> MSILTRWLLIPPVNARLIGRYRDYRRHGASAFSATLGCFWMILAWIFIPLEHPRWQRIRAEHKNLYPHINASRPRPLDPVRYLIQTCWLLIGASRKETPKPRRRAFSGLQNIRGRYHQWMNELPERVSHKTQHLDEKKELGHLSAGARRLILGIIVTFSLILALICVTQPFNPLAQFIFLMLLWGVALIVRRMPGRFSALMLIVLSLTVSCRYIWWRYTSTLNWDDPVSLVCGLILLFAETYAWIVLVLGYFQVVWPLNRQPVPLPKDMSLWPSVDIFVPTYNEDLNVVKNTIYASLGIDWPKDKLNIWILDDGGREEFRQFAQNVGVKYIARTTHEHAKAGNINNALKYAKGEFVSIFDCDHVPTRSFLQMTMGWFLKEKQLAMMQTPHHFFSPDPFERNLGRFRKTPNEGTLFYGLVQDGNDMWDATFFCGSCAVIRRKPLDEIGGIAVETVTEDAHTSLRLHRRGYTSAYMRIPQAAGLATESLSAHIGQRIRWARGMVQIFRLDNPLTGKGLKFAQRLCYVNAMFHFLSGIPRLIFLTAPLAFLLLHAYIIYAPALMIALFVLPHMIHASLTNSKIQGKYRHSFWSEIYETVLAWYIAPPTLVALINPHKGKFNVTAKGGLVEEEYVDWVISRPYIFLVLLNLVGVAVGIWRYFYGPPTEMLTVVVSMVWVFYNLIVLGGAVAVSVESKQVRRSHRVEMTMPAAIAREDGHLFSCTVQDFSDGGLGIKINGQAQILEGQKVNLLLKRGQQEYVFPTQVARVMGNEVGLKLMPLTTQQHIDFVQCTFARADTWALWQDSYPEDKPLESLLDILKLGFRGYRHLAEFAPSSVKGIFRVLTSLVSWVVSFIPRRPERSETAQPSDQALAQQGSARSSGRTGLEFEEFYPYDVPDYAADYKDDDDKRS;>MKRKLFWICAVAMGMSAFPSFMTQATPATQPLINAEPAVAAQTEQNPQVGQVMPGVQGADAPVVAQNGPSRDVKLTFAQIAPPPGSMVLRGINPNGSIEFGMRSDEVVTKAMLNLEYTPSPSLLPVQSQLKVYLNDELMGVLPVTKEQLGKKTLAQMPINPLFITDFNRVRLEFVGHYQDVCENPASTTLWLDVGRSSGLDLTYQTLNVKNDLSHFPVPFFDPRDNRTNTLPMVFAGAPDVGLQQASAIVASWFGSRSGWRGQNFPVLYNQLPDRNAIVFATNDKRPDFLRDHPAVKAPVIEMINHPQNPYVKLLVVFGRDDKDLLQAAKGIAQGNILFRGESVVVNEVKPLLPRKPYDAPNWVRTDRPVTFGELKTYEEQLQSSGLEPAAINVSLNLPPDLYLMRSTGIDMDINYRYTMPPVKDSSRMDISLNNQFLQSFNLSSKQEANRLLLRIPVLQGLLDGKTDVSIPALKLGATNQLRFDFEYMNPMPGGSVDNCITFQPVQNHVVIGDDSTIDFSKYYHFIPMPDLRAFANAGFPFSRMADLSQTITVMPKAPNEAQMETLLNTVGFIGAQTGFPAINLTVTDDGSTIQGKDADIMIIGGIPDKLKDDKQIDLLVQATESWVKTPMRQTPFPGIVPDESDRAAETRSTLTSSGAMAAVIGFQSPYNDQRSVIALLADSPRGYEMLNDAVNDSGKRATMFGSVAVIRESGINSLRVGDVYYVGHLPWFERLWYALANHPILLAVLAAISVILLAWVLWRLLRIISRRRLNPDNE[4x];>[2x]MTQFTQNTAMPSSLWQYWRGLSGWNFYFLVKFGLLWAGYLNFHPLLNLVFAAFLLMPLPRYSLHRLRHWIALPIGFALFWHDTWLPGPESIMSQGSQVAGFSTDYLIDLVTRFINWQMIGAIFVLLVAWLFLSQWIRITVFVVAILLWLNVLTLAGPSFSLWPAGQPTTTVTTTGGNAAATVAATGGAPVVGDMPAQTAPPTTANLNAWLNNFYNAEAKRKSTFPSSLPADAQPFELLVINICSLSWSDIEAAGLMSHPLWSHFDIEFKNFNSATSYSGPAAIRLLRASCGQTSHTNLYQPANNDCYLFDNLSKLGFTQHLMMGHNGQFGGFLKEVRENGGMQSELMDQTNLPVILLGFDGSPVYDDTAVLNRWLDVTEKDKNSRSATFYNTLPLHDGNHYPGVSKTADYKARAQKFFDELDAFFTELEKSGRKVMVVVVPEHGGALKGDRMQVSGLRDIPSPSITDVPVGVKFFGMKAPHQGAPIVIEQPSSFLAISDLVVRVLDGKIFTEDNVDWKKLTSGLHKQHRSPRTQMQ;>MASWSHPQFEKGSMRDIVDPVFSIGISSLWDELRHMPAGGVWWFNVDRHEDAISLANQTIASQAETAHVAVISMDSDPAKIFQLDDSQGPEKIKLFSMLNHEKGLYYLTRDLQCSIDPHNYLFILVCANNAWQNIPAERLRSWLDKMNKWSRLNHCSLLVINPGNNNDKQFSLLLEEYRSLFGLASLRFQGDQHLLDIAFWCNEKGVSARQQLSVQQQNGIWTLVQSEEAEIQPRSDEKRILSNVAVLEGAPPLSEHWQLFNNNEVLFNEARTAQAATVVFSLQQNAQIEPLARSIHTLRRQRGSAMKILVRENTASLRATDERLLLACGANMVIPWNAPLSRCLTMIESVQGQKFSRYVPEDITTLLSMTQPLKLRGFQKWDVFCNAVNNMMNNPLLPAHGKGVLVALRPVPGIRVEQALTLCRPNRTGDIMTIGGNRLVLFLSFCRINDLDTALNHIFPLPTGDIFSNRMVWFEDDQISAELVQMRLLAPEQWGMPLPLTQSSKPVINAEHDGRHWRRIPEPMRLLDDAVERSS[2x];>[2x]MMTISDIIEIIVVCALIFFPLGYLARHSLRRIRDTLRLFFAKPRYVKPAGTLRRTEKARATKK;>[2x]MAVLGLQGVRGGVGTTTITAALAWSLQMLGENVLVVDACPDNLLRLSFNVDFTHRQGWARAMLDGQDWRDAGLRYTSQLDLLPFGQLSIEEQENPQHWQTRLSDICSGLQQLKASGRYQWILIDLPRDASQITHQLLSLCDHSLAIVNVDANCHIRLHQQALPDGAHILINNFRIGSQVQDDIYQLWLQSQRRLLPMLIHRDEAMAECLAAKQPVGEYRSDALAAEEILTLANWCLLNYSGLKTPVGSKS;>MGSSHHHHHHHHAAGSNNNEPDTLPDPAIGYIFQNDIVALKQAFSLPDIDYADISQREQLAAALKRWPLLAEFAQQK[2x]

Bacterial cellulosic polymers constitute a prevalent class of biofilm matrix exopolysaccharides that are synthesized by several types of bacterial cellulose secretion (Bcs) systems, which include conserved cyclic diguanylate (c-di-GMP)-dependent cellulose synthase modules together with diverse accessory subunits. In E. coli, the biogenesis of phosphoethanolamine (pEtN)-modified cellulose relies on the BcsRQABEFG macrocomplex, encompassing inner-membrane and cytosolic subunits, and an outer membrane porin, BcsC. Here we present cryo-EM structures of the E. coli Bcs macrocomplex positioning all seven BcsRQABEFG partners and multiple c-di-GMP-binding sites.

Here we locally refined the structure of the crownless Bcs macrocomplex complex to an average resolution of 2.85 Å, visualizing all interaction interfaces and coordinated nucleotide co-factors. An assymetric BcsR2Q2 complex is recruited to the membrane complex via BcsE’s C-terminal elongated tails, where both BcsQ copies interact with the synthase’s PilZ module and adopt the nucleotide-driven sandwich dimer conformation characteristic for the SIMIBI (SIgnal recognition particle, MinD, and BioD) family of protein-sorting NTPases to which BcsQ belongs. Importantly, whereas one of the BcsR protomers is solvent-exposed and features an unresolved N-terminal domain, the other BcsR copy also interacts with the back of the BcsA catalytic module. Contrary to the crystallized states where BcsRNTD can adopt a β-hairpin conformation that threads onto the surface of dimeric BcsQ, here residues D21-S30 fold into an N-proximal α-helix (αN) that U-turns into an extended linker before adopting the V-shaped C-terminal domain onto the BcsQ dimer interface. The resulting N-terminal hairpin nestles into a hydrophobic BcsAGT pocket via a L25-F29-L31-I34 plug at the tip and a I22:Y36 stabilizing interaction at the base. The BcsAPilZ domain orientation is further stabilized by interactions between the β4–β5 connecting loop of the PilZ barrel and N-proximal residues from BcsR-αC1, as well as by an extensive interface with the underlying BcsQ protomer (682 Å buried with a free energy gain of −4.1 kcal/mol). On the other side of the β-barrel, an intercalated c-di-GMP dimer is found coordinated between the arginines from the canonical R696RxxR motif in the N-proximal PilZ domain linker, the active site gating loop is unstructured, and the active site is substrate-accessible. In the c-di-GMP-saturated macrocomplex, one BcsEGGDEF* copy adopts an overall interaction interface consistent with the previously reported crystallized states and contacts BcsAGT via its REC* module. The second BcsEGGDEF*, on the other hand, positions above the BcsQ dimer interface and is further stabilized by the β-strand connecting loops at the bottom of the BcsAPilZ domain barrel.> RVEKAKQKSAQQELKQRQRA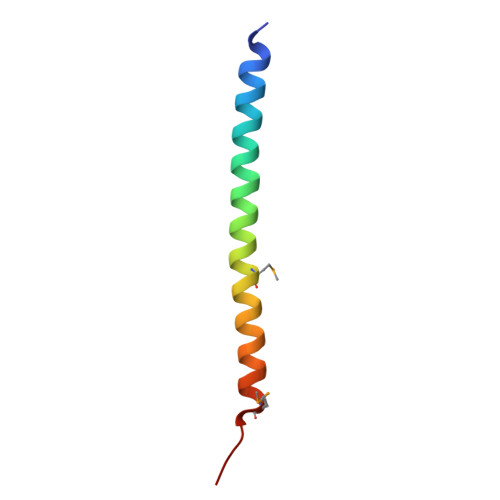EIYALNRVMTELEQQQFDEFCKQMQPPGE> KETA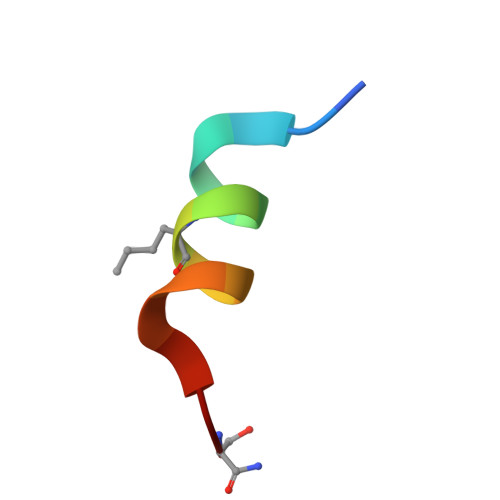AAKLERQHLDS> SMADGNEDLRADDLPGPAFESYESMELACPAERSGHVAVSDGRHMFVWGGYKSNQVRGLYDFYLPREELWIYNMETGRWKKINTEGDVPPSMSGSCAVCVDRVLYLFGGHHSRGNTNKFYMLDSRSTDRVLQWERIDCQGIPPSSKDKLGVWVYKNKLIFFGGYGYLPEDKVLGTFEFDETSFWNSSHPRGWNDHVHILDTETFTWSQPITTGKAPSPRAAHACATVGNRGFVFGGRYRDARMNDLHYLNLDTWEWNELIPQGICPVGRSWHSLTPVSSDH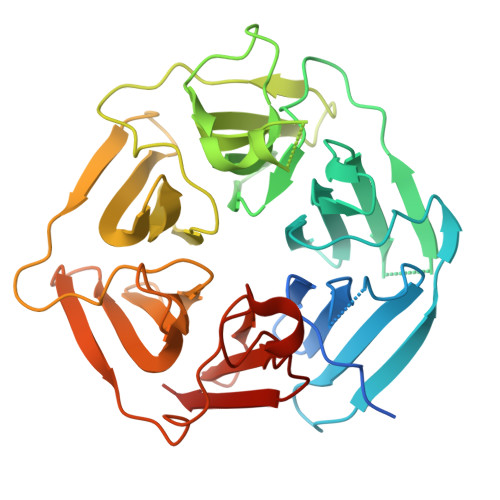LFLFGGFTTDKQPLSDAWTYCISKNEWIQFNHPYTEKPRLWHTACASDEGEVIVFGGCANNLLVHHRAAHSNEILIFSVQPK>[2x]MEEPPLLPGENIKDMAKDVTYICPFTGAVRGTLTVTNYRLYFKSMERDPPFVLDASLGVINRVEKIGGASSRGENSYGLETVCKDIRNLRFAHKPEGRTRRSIFENLMKYAFPVSNNLPLFAFEYKEVFPENGWKLYDPLLEYRRQGIPNESWRITKINERYELCDTYPALLVVPANIPDEELKRVASFRSRGRIPVLSWIHPESQATITRCSQPMVGVSGKRSKEDEKYLQAIMDSNAQSHKIFIFDARPSVNAVANKAKGGGYESEDAYQNAELVFLDIHNIHVMRESLRKLKEIVYPNIEETHWLSNLESTHWLEHIKLILAGALRIADKVESG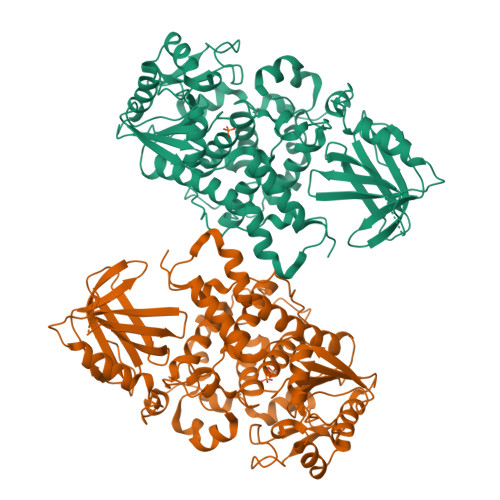KTSVVVHSSDGWDRTAQLTSLAMLMLDGYYRTIRGFEVLVEKEWLSFGHRFQLRVGHGDKNHADADRSPVFLQFIDCVWQMTRQFPTAFEFNEYFLITILDHLYSCLFGTFLCNSEQQRGKENLPKRTVSLWSYINSQLEDFTNPLYGSYSNHVLYPVASMRHLELWVGYYIRWNPRMKPQEPIHNRYKELLAKRAELQKKVEELQREISNRSTSSSERASSPAQCVTPVQTVV> MELKHSISDYTEAEFLQLVTTICNADTSSEEELVKLVTHFAEMTEHPSGSDLIYYPKEGDDDSPSGIVNTVKQWRAANGKSGFKQG;> MESKRNKPGKATGKGKPVGDKWLDDAGKDSGAPIPDRIADKLRDKEFKSFDDFRKAVWEEVSKDP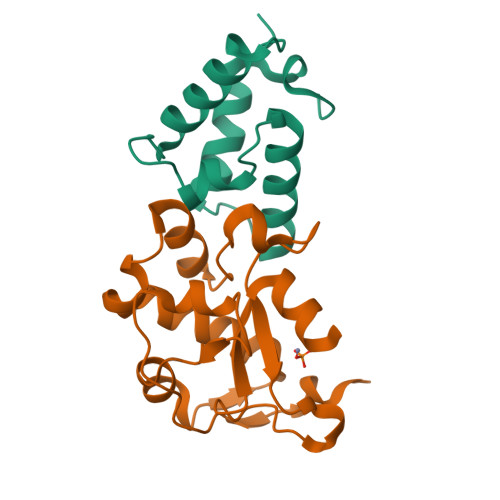ELSKNLNPSNKSSVSKGYSPFTPKNQQVGGRKVYELHHDKPISQGGEVYDMDNIRVTTPKRHIDIHRGK Fumarate addition is accomplished by X-succinate synthases (XSSs), which are members of the glycyl radical enzyme (GRE) superfamily. The denitrifying betaproteobacterium Azoarcus sp. strain HxN1 has been shown to degrade saturated alkanes, including n-hexane, n-heptane, and n-octane. A homolog of the catalytic BSS subunit has previously been identified in strain HxN1 and is thought to catalyze the addition of fumarate to these alkanes at the C2 position, thus producing (1-methylalkyl)succinates. As such, this homolog is referred to as (1-methylalkyl)succinate synthase (MASS).

Here, we present a structure of the MASS complex solved by single particle cryogenic electron microscopy (cryo-EM). We were able to build a molecular model for a MASSα2βγ2δ complex using the high-resolution EM map. One MASSα protomer is more complete than the other (MASSα: residues 15 to 839, MASSα′: residues 36 to 677, missing density for loops 375 to 380 and 588 to 593). Both MASSα and MASSα' bind one MASSγ protomer in a similar manner as BSSα binds BSSγ. One protomer of MASSβ and one of MASSδ are also bound to MASSα; however, there is no density for either of these subunits on MASSα′. Comparison of the α-subunits reveals that the GRD is completely disordered when the β- and δ-subunits are absent, consistent with increased GRD mobility in the absence of these subunits. However, instead of finding density for the predicted [4Fe–4S] cluster, the density was consistent with the presence of a single Fe ion. Furthermore, when we compare the overall fold of MASSδ to that of other known proteins, we observe that MASSδ has a rubredoxin-like fold, a fold associated with the binding of a single Fe ion [Fig. 4B (33)]. Like BSS, one carboxylate group of fumarate is held in place by an oxyanion hole created by the Cys loop whereas the other carboxylate group forms an electrostatic interaction with an active site Arg residue (Arg508 in BSS, Arg492 in MASS). In BSS, BSSβ is the only barrier to toluene entering the active site; however, in MASS, Trp185 blocks the substrate channel as well. Specifically, we propose that MASSβ gates substrate entry, whereas MASSδ regulates GRD conformational changes.

>[2x]MGSSHHHHHHSQMTATSTLSKTDLKNCETVEELRENQQWWWLAERERSARLDYLRKATWKKGALGGNYFDGIRLDLEYPTLFTEAWKKYPNDPSMLRRAKATAYVLDNISIFITDSAQLVGYVGSAPHTIAWRVDGASTVNSEVYNEPGIHAEPEAESLKKVAEINSYWNGQTAVDKVGRLIDPEDAVKFFSGAIGWGTPSSAFGYSGKNFEYFMKGDRAFSQIIAEIDEKIDEAEEATIGTPSPHILPLYDKLNNWHAMKLVLEAAIRFAGRYARLARVMAAKETDEQRKKELLRVAETCERVPANPPRNLQESLQYEHFVQVLARYEAHEGAWPSRPDYYHGPLYAKDVEVEKNITESEAIDLVGEYMIRCSEYGSFSPRYMREGLQGVTGTFVWTLGGVNQDGTDACNGMTIALLKAARLVRVANPTFGFRWHPKVSNEVLRECFECIRQGLGYPTLRNDPVLIQNTMHWYGHPLEEARTWVHMACMSPNPTTKHGTSPFRMASATMNSAKTIEYVLHNGYDRVVNMQMGPKTGDAREIKDFEDLFERWTVQLKWLMNLLVRTVNLGRFKDPEFFGRPFLSAITERAVEHGIDAVSPEGERGNAWVTAFTWIENVDSMAAIKKLVFDDKKYTMSQLIDALEAEWDGYEQMRLDFVKNGPKWGNDDDYVDDIMLRCLSVAAEHSRNIQCTSGNCWPILPENVSGNIHYANIVGALPNGRRRGDALYDGGVSPGPGLDKAGPTAVLKSVGKIDHVNQGRSFLLNQRLSPTQLAGDKGFQLWNSYVRTWAELGIDHIQFNVISDKVLRAAQNDPEGYQEVIVRVAGYSAHFIDISRKTQDNIIQRTVQGLGENLYFQG;> MSRRDEWKKLQEEMTRDGGEIKSLETVPEQACGICLNFTDNAYGSDGRGSCNVLKAGSNISLPDVIITRSGENGYITFFNSDAKYCPNFERMKLIDTDGHECADPISRRVQRQLSSIKKS;>STCKECRNYFPINEEASRGDCVRRISDERQSYYTARPTTEAAKCEGCSDYLENTRTAKAH[2x];> MKCTECGHEAEVMKFRYHYNPRIDASLSLRQCPECQAVVTVDELKREVLGRMHNGDDPWGKSAGIENLAEG>[3x]HGEKSQQAFLRMRTLNWYDVQWSKTTVNVNEEMVLSGKVHVFSAWPQAVAN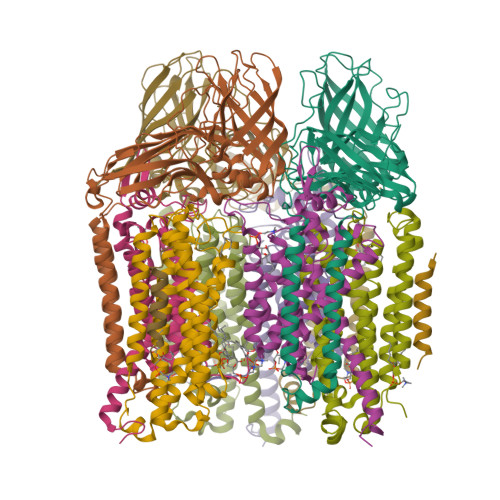PRVSFLNAGEPGPVLVRTAQFIGEQFAPRSVSLEIGKDYAFSINLRGRRAGRWHVHAQINVEGGGPIIGPGQWIEIKGDMKDFTDPVTLLDGSTVDLEHYGISRVYAWHLPWMAVGAAWIFFWFVRKGIITSYIRVAEGKADDVIGDDDRRIGAIVLALTILATIVGYAVTNSTFPRTIPLQAGLQKPLTPIETEGTVGVGKENVTTELNGGVYKVPGRELTINVKVKNNTSQPLRLGEYTAAGLRFLNPDVFTTKPDFPDYLLADRGLSVDATPIAPGEAKEIVVKIQDARWDIERLSDLAYDTDSQIGGLLFFFSPDGKRYASEIGGPVIPKFVA;>[3x]AVGPFNSVAEAAGCVQTVDWMLLVLLFFAVLGGYHVHFMLTAGDWDFWVDWKDRRMWPTVVPILGVTFCAASQAFWWVNFRLPFGAVFAALGLLIGEWINRYVNFWGWTYFPISLVFPSALIVPAIWLDVILLLSGSYVITAVVGSLGWGLLFYPNNWPAIAAFHQATEQHGQLMTLADLIGFHFVRTSMPEYIRMVERGTLRTFGKDVVPVAAFFSGFVSMMVYFLWWFMGRWYSTTKVIDTI;>[3x]ESVVDLRGMWIGLVLLNVFYLIVRIYEQVFGWRAGLDSFAPEFQTYWMSILWTEIPLELVSGLGLAGYLWKTRDRNVDAVTPREEMRRLVVLVQWLVVYGIAIYWGASFFTEQDGTWHMTVIRDTDFTPSHIIEFYMSYPIYSVIAVGAFFYAKTRIPYFAHGYSLAFLIVAIGPFMIIPNVGLNEWGHTFWFMEELFVAPLHWGFVFFGWMALGVFGVVLQILMRIHALVGKEGVKLLTE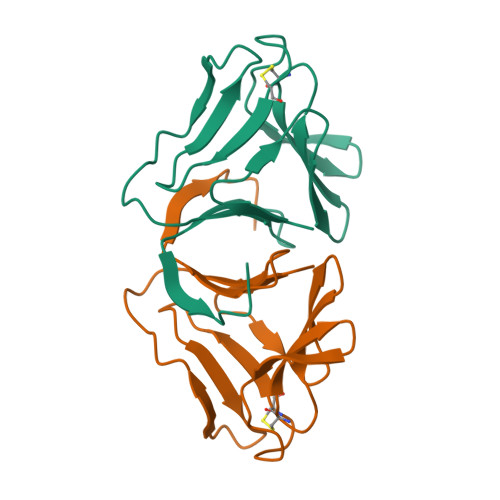>[4x]VNSLSSPNSLFTGHSLEVGPSYRLIMQGDCNFVLYDSGKPVWASNTGGLGSGCRLTLHNNGNLVIYDQSNRVIWQTKTNGKEDHYVLVLQQDRNVVIYGPVVWATGSGPA>[16x]GSHMTGELEVKNMDMKPGSTLKITGSIADGTDGFVINLGQGTDKLNLHFNPRFSES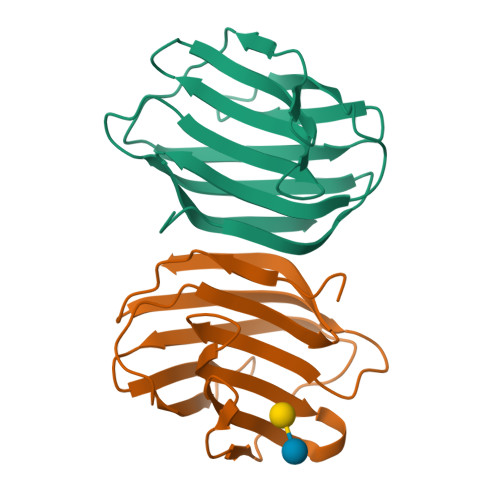TIVCNSLDGSNWGQEQREDHLCFSPGSEVKFTVTFESDKFKVKLPDGHELTFPNRLGHSHLSYLSVRGGFNMSSFKLK> MNDDRETPPKRKPGEDDTLFDIDFLDDTTSHSGSRSKVTNSHANANYIPPSHVLPEETIDLDADDDNIENDVHENLFMSNNHDDQTSWNANRFDSDAYQPQSLRAVKPPGLFARFGNGLKNAFTFKRKKGPESFEMNHYNAVTNNELDDNYLDSRNKFNIKILFNRYILRKNVGDAEGNGEPRVIHINDSLANSSFGYSDNHISTTKYNFATFLPKFLFQEFSKYANLFFLCTSAIQQVPHVSPTNRYTTIGTLLVVLIVSAMKECIEDIKRANSDKELNNSTAEIFSEAHDDFVEKRWIDIRVGDIIRVKSEEPIPADTIILSSSEPEGLCYIETANLDGETNLKIKQSRVETAKFIDVKTLKNMNGKVVSEQPNSSLYTYEGTMTLNDRQIPLSPDQMILRGATLRNTAWIFGLVIFTGHETKLLRNATATPIKRTAVEKIINRQIIALFTVLIVLILISSIGNVIMSTADAKHLSYLYLEGTNKAGLFFKDFLTFWILFSNLVPISLFVTVELIKYYQAFMIGSDLDLYYEKTDTPTVVRTSSLVEELGQIEYIFSDKTGTLTRNIMEFKSCSIAGHCYDDKIPEDKTATVEDGIEVGYRKFDDLKKKLNDPSDEDSPIINDFLTLLATCHTVIPEFQSDGSIKYQAASPDEGALVQGGADLGYKFIIRKPNSVTVLLEETGEEKEYQLLNICEFNSTRKRMSAIFR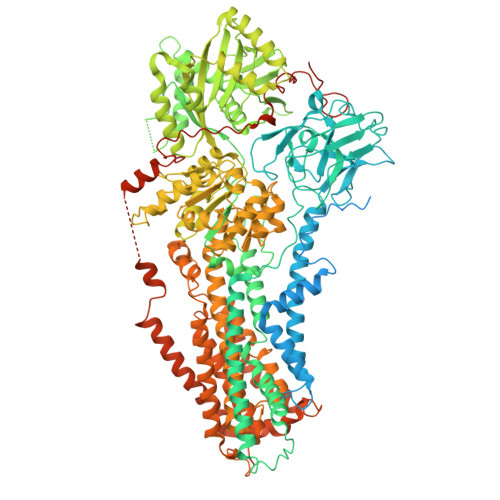FPDGSIKLFCKGADTVILERLDDEANQYVEATMRHLEDYASEGLRTLCLAMRDISEGEYEEWNSIYNEAATTLDNRAEKLDEAANLIEKNLILIGATAIEDKLQDGVPETIHTLQEAGIKIWVLTGDRQETAINIGMSCRLLSEDMNLLIINEETRDDTERNLLEKINALNEHQLSTHDMNTLALVIDGKSLGFALEPELEDYLLTVAKLCKAVICCRVSPLQKALVVKMVKRKSSSLLLAIGDGANDVSMIQAAHVGVGISGMEGMQAARSADIAVGQFKFLKKLLLVHGSWSYQRISVAILYSFYKNTALYMTQFWYVFANAFSGQSIMESWTMSFYNLFFTVWPPFVIGVFDQFVSSRLLERYPQLYKLGQKGQFFSVYIFWGWIINGFFHSAIVFIGTILIYRYGFALNMHGELADHWSWGVTVYTTSVIIVLGKAALVTNQWTKFTLIAIPGSLLFWLIFFPIYASIFPHANISREYYGVVKHTYGSGVFWLTLIVLPIFALVRDFLWKYYKRMYEPETYHVIQEMQKYNISDSRPHVQQFQNAIRKVRQVQRMKKQRGFAFSQAEEGGQEKIVRMYDTTQKRGKYGELQDASANPFNDNNGLGSNDFESAEPFIENPFADGNQNSNRFSSSRDDISFDI> HHHHHHMSSGKNAPKTGGGAKGNNASPAGSGNTKNNGA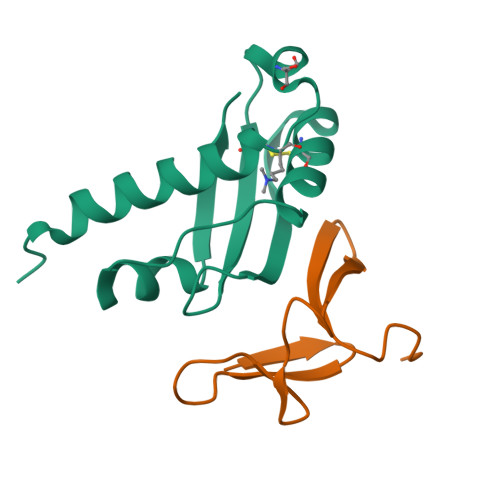SGADINNYAGQIKSAIESKFYDASSYAGKTCTLRIKLAPDGMLLDIKPEGGDPALCQAALAAAKLAKIPKPPSQAVYEVFKNAPLDFKP;> GSKPGDSYNTPWGKVIINAAGQPTMNGTVMTADNSSMVPYGRGFTRVLNSLVNNPVSHHHHHH>SNAMKNYYSSNPTFYLGIDCIIFGFNEGEISLLLLKRNFEPAMGEWSLMGGFVQKDESVDDAAKRVLAELTGLENVYMEQVGAFGAIDRDPGERVVSIAYYALININEYDRELVQKHNAYWVNINELPALIFDHPEMVDKAREMMKQKASVEPIGFNLLPKLFTLSQLQSLYEAIYGEPMDKRNFRKRVAEMDFIEKTDKIDKLGSKRGAALYKFNGKAYRKDPKFKL[4x]

In this study we identified and characterized a novel L-arabinose-responsive transcription factor found in the Bacteroides species, which belongs to the NrtR family of Nudix-related transcriptional regulators. The NrtR family transcription factors are characterized by an N-terminal Nudix hydrolase-like effector-binding domain and a C-terminal DNA-binding domain. In this work, genome-scale regulon inference using the comparative genomics approach revealed that the NrtR family AraR regulators in Bacteroides and Prevotella spp. control not only the L-arabinose catabolic operons, but also several other gene loci involved in the utilization of arabinose-containing polysaccharides. The predicted AraR-regulated operons are involved in the uptake and catabolism of L-arabinose and the decomposition of arabinose-containing polysaccharides (e.g., arabinan, arabinoxylan, pectic galactan) to oligosaccharides, their translocation into the periplasm, and further hydrolysis.

We determined the structures of full-length apo–BtAraR protein, its complex with a specific DNA duplex, and its complex with the L-arabinose effector. The solved structures provide a first view of the structural mechanism underlying the regulatory function of the L-arabinose-binding Nudix domain. The Nudix signature motif GX5-EX7REUXEEXGU (where U is a hydrophobic residue and X is any residue) is strictly conserved in all known active Nudix hydrolases, but it is impaired in the NrtR regulators of NAD metabolism, several of which are known to be enzymatically inactive. Similarly to NrtR regulators, the Nudix signature motif is not conserved in the AraR proteins from Bacteroidetes, where two or three glutamate residues are substituted with other amino acids. These observations suggest that AraR regulators are also enzymatically inactive and utilize their Nudix hydrolase-like domains for ligand binding.Here, we elucidated the molecular mechanism underlying the function and regulation of P. fluorescens LapD, a transmembrane receptor essential for biofilm formation in this strain. As c-di-GMP levels change LapD switches between two states: the dinucleotide-unbound off state that retards stable biofilm formation by facilitating the secretion of the cell surface adhesin LapA, and the c-di-GMP-bound on state that supports cell adhesion by preventing the release of LapA from the outer membrane. Binding of c-di-GMP to the LapD EAL domain is relayed to the periplasmic output domain through an inside-out signaling mechanism that utilizes a juxtamembrane HAMP domain, a relay module often found in bacterial transmembrane receptors. Here, we present three crystal structures of LapD from P. fluorescens that provide models for the c-di-GMP-unbound cytoplasmic domain lacking only the HAMP domain, a c-di-GMP-bound EAL domain dimer, and the periplasmic domain.

The crystal structure of LapDEAL bound to c-di-GMP (residues 399–648; LapDEAL•c-di-GMP) was solved by molecular replacement using the EAL domain from apo-LapDdual as the search model. We obtained crystals in two independent conditions, yielding two different crystal forms (space group C2221, two molecules per asymmetric unit; and space group P6522, one molecule per asymmetric unit). While the majority of the crystal packing contacts were different, both crystal forms maintained a common dimer of EAL domains, and the resulting structures superimposed almost perfectly (rmsd of 0.6 Å over all atoms). The crystal structure of dimeric, c-di-GMP-bound EAL domains provides insight into the conformational changes resulting from dinucleotide binding. c-di-GMP binding did not alter the overall conformation of the EAL domain observed in the apo-LapDdual structure (rmsd of 0.6 Å over all atoms), consistent with the lack of major conformational changes upon dinucleotide binding to the EAL domains of YkuI, TDB1265, and FimX. Minor changes in the dinucleotide-binding pocket are confined to four c-di-GMP-coordinating residues that adopt an alternate side chain rotamer conformation. The most notable conformational change in LapDEAL upon c-di-GMP binding occurs in the switch loop. In contrast, the switch loop adopts a conformation in the c-di-GMP-bound structure positioning F566 so that it can participate in homodimerization. Most importantly, dimerization of the c-di-GMP-bound EAL domains is incompatible with the conformation observed in the crystals of apo-LapDdual. The surface occupied by the S helix overlaps significantly with the homodimerization interface, which indicates that dinucleotide-induced conformational changes will include the displacement of the GGDEF domain and the S helix.

>[2x]QSLVADVGDDHHAWHRLLDQALNQRRFELFFQPVVAAQDTQLVLHYKVLSRLLDEQGQTIPAGRFLPWLERFGWTARLDRLMLERVLEQMAGHEESLALNLSSATLADPQALNKVFEILRAHSNLGARLTLEIGEEQLPEQAVLEQLTRRLRELGFSLSLQRFGGRFSMIGNLARLGLAYLKIDGSYIRAIDQESDKRLFIEAIQRAAHSIDLPLIAERVETEGELSVIREMGLYGVQGQLFGEPKPWG N-[(1E)-PYRIDIN-2-YLMETHYLENE]-N-[4-(4-{[(1E)-PYRIDIN-2-YLMETHYLENE]AMINO}BENZYL)PHENYL]AMINE 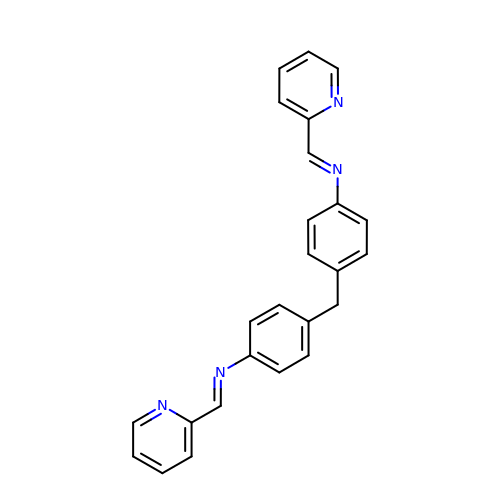| C25 H20 N4 | OMZVNZJNZUGOJK-UOSOPFLXSA-N Here we systematically reconstruct a part of the metabolism of the GRM3 of Rhodopseudomonas palustris BisB18 by functionally and structurally characterizing three core enzymes, and by reconstituting the reaction sequence in vitro. Furthermore, we show that the acylating aldehyde dehydrogenase (AldDH), encoded within the GRM gene cluster, preferentially uses propionaldehyde as substrate. In summary, characterization of the GRM3 AldDH leads to a revised and detailed reaction mechanism for the ubiquitous (present in all three domains of life) family of acylating aldehyde dehydrogenases. These enzymes take part in numerous pathways including fermentations, detoxifications, other catabolic and central carbon metabolic processes.

When AldDH was crystallized at pH 4.8 with propionyl-CoA, we obtained crystals with triclinic P 1 symmetry, diffracting to a resolution of 2.5 Å. We used the same condition to co-crystallize AldDH with NAD+. These crystals had monoclinic P21 symmetry, diffracted to a resolution of 2.3 Å and exhibited twinning (twin fraction of 37%). Electron density in the active sites allowed the fitting of NAD+. Interestingly, both co-substrates, NAD+ and (propionyl-)CoA, occupy a similar position in the two structures but with their adenine rings pointing in opposite directions. This was also reported for crystal structures of the AldDH homolog from C. phytofermentans, and is consistent with a proposed bi-uni-uni-uni ping pong mechanism, in which the aldehyde would bind to the active site together with NAD+. Subsequently NADH is released from the active site before CoA can bind and the final product, acyl-CoA, is released again. A conserved glutamate (Glu419) forms hydrogen bonds to the nicotinamide ribose, which appears to facilitate the correct positioning of NAD+ for the hydride transfer.

>MAWSHPQFEKGHMNDANIADVVTKVLGEYGAPGAVSVAALTAKSPDGKSNSSADADVVARMVAKAIRDHAGTAQPSGNAATSSAAVSDGVFETMDAAVEAAALAQQQYLLCSMSDRARFVQGIRDVILNQDTLEKMSRMAVEETGMGNYEHKLIKNRLAGEKTPGIEDLTTDAFSGDNGLTLVEYSPFGVIGAITPTTNPTETIVCNSIGMLAAGNSVVFSPHPRARQVSLLLVRLINQKLAALGAPENLVVTVEKPSIENTNAMMAHPKVRMLVATGGPAIVKAVLSTGKKAIGAGAGNPPVVVDETANIEKAACDIVNGCSFDNNLPCVAEKEIIAVAQIADYLIFNLKKNGAYEIKDPAVLQQLQDLVLTAKGGPQTKCVGKSAVWLLSQIGISVDASIKIILMEVPREHPFVQEELMMPILPLVRVETVDDAIDLAIEVEHDNRHTAIMHSTDVRKLTKMAKLIQTTIFVKNGPSYAGLGAGGEGYSTFTIAGPTGEGLTSAKSFARRRKCVMVEALNIR[8x]>DGVGNASGDWHCDSTWSEGRVTTTSTRTWVLPTYNNHLYLRIGTTANSNTYNGFSTPWGYFDFNRFHCHFSPRDWQRLINNNWGLRPKSMRVKIFNIQVKEVTTSNGETTVANNLTSTVQIFADSTYELPYVMDAGQEGSFPPFPNDVFMVPQYGYCGVVTGKNQNQTDRNAFYCLEYFPSQMLRTGNNFEVSYQFEKVPFHSMYAHSQSLDRMMNPLLDQYLWHLQSTTTGNSLNQGTATTTYGKITTGDFAYYRKNWLPGACIKQQKFSKNANQNYKIPASGGDALLKYDTHTTLNGRWSNMAPGPPMATAGAGDSDFSNSQLIFAGPNPSGNTTTSSNNLLFTSEEEIATTNPRDTDMFGQIADNNQNATTAPHIANLDAMGIVPGMVWQNRDIYYQGPIWAKVPHTDGHFHPSPLMGGFGLKHPPPQIFIKNTPVPANPNTTFSAARINSFLTQYSTGQVAVQIDWEIQKEHSKRWNPEVQFTSNYGTQNSMLWAPDNAGNYHELRAIGSRFLTHHL[60x]

Adeno-associated viruses (AAV) are single-stranded DNA packaging viruses of the Parvoviridae and belong to the genus Dependoparvovirus. The virions of the AAVs are composed of non-enveloped capsids with T = 1 icosahedral symmetry and diameters of ≈260 Å. They are assembled from 60 viral proteins (VPs): VP1 (≈82 kDa), VP2 (≈73 kDa), and VP3 (≈61 kDa) in an approximate 1:1:10 ratio. In this study, the structures of the AAV7, AAV11, AAV12, and AAV13 capsids were determined by cryo-EM in an effort to complete the panel of available structures for the defined AAV serotypes.

For AAV11 and AAV12, the closest related AAV serotype is AAV4 based on VP1 or VP3 amino acid sequence ranging from 78 to 81% aa sequence identity. In contrast, major structural variabilities (vs. AAV2) were seen in VR-I, VR-III, VR-IV, VR-V, VR-VI, VR-VII, and VR-IX for AAV11 and AAV12. Most notably is the 5 aa insertion in VR-V for both AAV11 and AAV12, relative to AAV2, but also to AAV7 and AAV13. In addition, both AAV serotypes possess a single aa insertion in VR-IV and display a different conformation to the other AAV serotypes with the apex of the loop positioned over part of VR-V. This subloop of VR-V and the alternative conformation of VR-IV are responsible for the broader appearance of the 3-fold protrusions of the AAV11 and AAV12 capsids. For AAV12, HSPG and sialic acids were excluded as a receptor, and no binding to the available glycans on an array was shown. An interesting difference between AAV4, AAV11, and AAV12 for AAV vector production is the requirement for the assembly activating protein (AAP) for capsid assembly. While AAV12 is dependent on the presence of AAP, AAV4 and AAV11 are not. While the VP structures of empty and full capsids were largely identical, some alternative side-chain orientations, e.g., histidine 230 (AAV7 numbering), were observed. In the AAV serotype structures determined in this study, the histidine side chain preferred the “left” orientation in full capsids. In contrast, both orientations are equally adopted in empty capsids, except for AAV12, where the right orientation appears to be favored.> GQMGEGFNWEIEQKMDSSTNNGILKTKYGFDNLYDTVISVSTSNGNDINELDDPEHTDANDRVIERLRKENLKFDPEYYVSEYMTHKYGNEEDLEINGIKELLKFTPSIVKQYLQWYKDSTNPNLVMPIEFTDEEQKQMQDNLPKKSYLVEDIKPLYVTILSVLFSYVFEQIENEGTHTTESAWTMGKLCPQISFLDQQLKQVNELQDGMKEISKVNKDSSLIKIAIITGIRRALSYPLHRNYDLAMKAWTFVYYILRGGKRLVIRALLDIHETFRFHDVYYVYDKVLLDDLTAWFISQ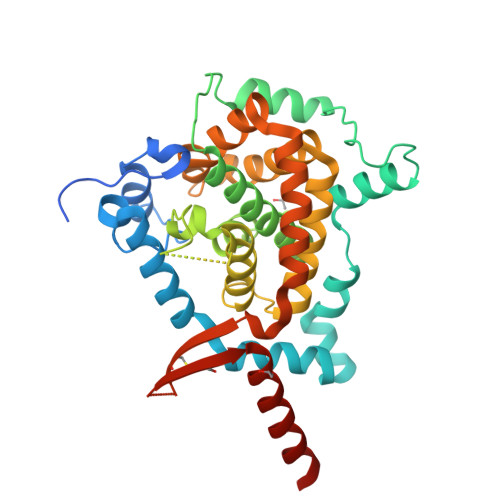GSENVIRSLALEMRKEQESLSKQDIEFECIASFNEQTGEPEWETLNIREMEILAESEYREQQQNPQ>MRGSHHHHHHGSSKKINGFEVLGEVAWLWASSPLHRKWPLSLLAINVLPAIESNQYVLLKRDGFPIAFCSWANLNLENEIKYLDDVASLVADDWTSGDRRWFIDWIAPFGDSAALYKHMRDNFPNELFRAIRVDPDSRVGKISEFHGGKIDKKLASKIFQQYH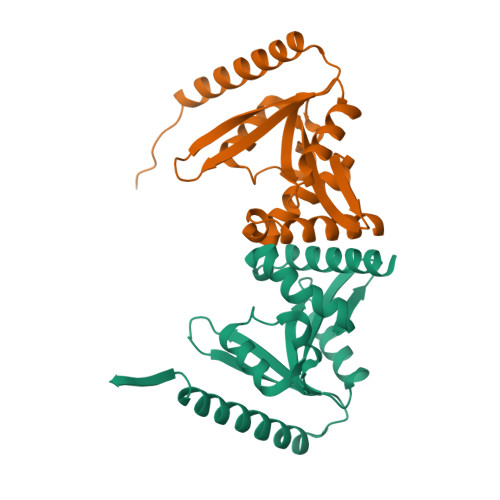FELMSELKNKQNFKFSLVNS[4x]cladosporin | C16 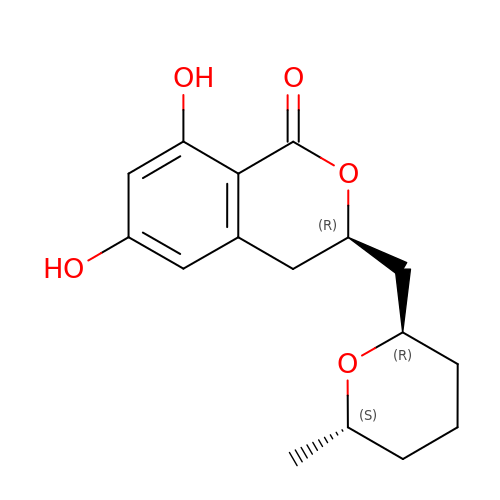H20 O5 | WOMKDMUZNBFXKG-ZWKOPEQDSA-N>[2x]MLDSKLKAPVFTVRTQGREYGEFVLEPLERGFGVTLGNPLRRILLSSIPGTAVTSVYIEDVLHEFSTIPGVKEDVVEIILNLKELVVRFLNPSLQTVTLLLKAEGPKEVKARDFLPVADVEIMNPDLHIATLEEGGRLNMEVRVDRGVGYVPAEKHGIKDRINAIPVDAVFSPVRRVAFQVEDTRLGQRTDLDKLTLRIWTDGSVTPLEALNQAVEILREHLTYFSNPQAAAVAAPEEAKEPEAPPEQEEELDLPLEELGLSTRVLHSLKEEGIESVRALLALNLKDLKNIPGIGERSLEEIKEALEKKGFTLKE;> MEIKRFGRIREVIPLPPLTEIQVESYRRALQADVPPEKRENVGIQAAFRETFPIEEEDKGKGGLVLDFLEYRLGEPPFPQDECREKDLTYQAPLYARLQLIHKDTGLIKEDEVFLGHIPLMTEDGSFIINGADRVIVSQIHRSPGVYFTPDPARPGRYIASIIPLPKRGPWIDLEVEPNGVVSMKVNKRKFPLVLLLRVLGYDQETLARELGAYGELVQGLMDESVFAMRPEEALIRLFTLLRPGDPPKRDKAVAYVYGLIADPRRYDLGEAGRYKAEEKLGIRLSGRTLARFEDGEFKDEVFLPTLRYLFALTAGVPGHEVDDIDHLGNRRIRTVGELMTDQFRVGLARLARGVRERMLMGSEDSLTPAKLVNSRPLEAAIREFFSRSQLSQFKDETNPLSSLRHKRRISALGPGGLTRERAGFDVRDVHRTHYGRICPVETPEGANIGLITSLAAYARVDELGFIRTPYRRVVGGVVTDEVVYMTATEEDRYTIAQANTPLEGNRIAAERVVARRKGEPVIVSPEEVEFMDVSPKQVFSVNTNLIPFLEHDDANRALMGSNMQTQAVPLIRAQAPVVMTGLEERVVRDSLAALYAEEDGEVAKVDGNRIVVRYEDGRLVEYPLRRFYRSNQGTALDQRPRVVVGQRVRKGDLLADGPASENGFLALGQNVLVAIMPFDGYNFEDAIVISEELLKRDFYTSIHIERYEIEARDTKLGPERITRDIPHLSEAALRDLDEEGVVRIGAEVKPGDILVGRTSFKGESEPTPEERLLRSIFGEKARDVKDTSLRVPPGEGGIVVRTVRLRRGDPGVELKPGVREVVRVYVAQKRKLQVGDKLANRHGNKGVVAKILPVEDMPHL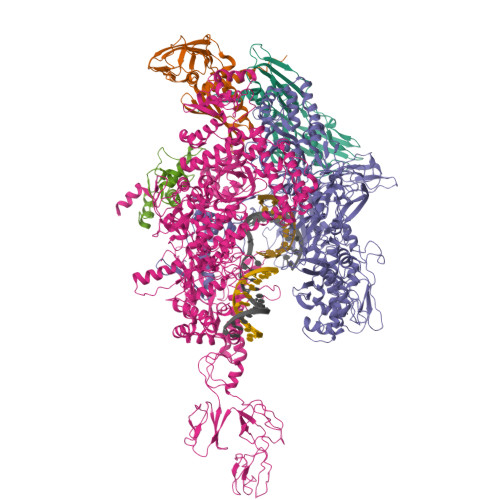PDGTPVDVILNPLGVPSRMNLGQILETHLGLAGYFLGQRYISPIFDGAKEPEIKELLAQAFEVYFGKRKGEGFGVDKREVEVLRRAEKLGLVTPGKTPEEQLKELFLQGKVVLYDGRTGEPIEGPIVVGQMFIMKLYHMVEDKMHARSTGPYSLITQQPLGGKAQFGGQRFGEMEVWALEAYGAAHTLQEMLTLKSDDIEGRNAAYEAIIKGEDVPEPSVPESFRVLVKELQALALDVQTLDEKDNPVDIFEGLASKR;> MKKEVRKVRIALASPEKIRSWSYGEVEKPETINYRTLKPERDGLFDERIFGPIKDYECACGKYKRQRFEGKVCERCGVEVTKSIVRRYRMGHIELATPAAHIWFVKDVPSKIGTLLDLSATELEQVLYFSKYIVLDPKGAILNGVPVEKRQLLTDEEYRELRYGKQETYPLPPGVDALVKDGEEVVKGQELAPGVVSRLDGVALYRFPRRVRVEYVKKERAGLRLPLAAWVEKEAYKPGEILAELPEPYLFRAEEEGVVELKELEEGAFLVLRREDEPVATYFLPVGMTPLVVHGEIVEKGQPLAEAKGLLRMPRQVRAAQVEAEEEGETVYLTLFLEWTEPKDYRVQPHMNVVVPEGARVEAGDKIVAAIDPEEEVIAEAEGVVHLHEPASILVVKARVYPFEDDVEVSTGDRVAPGDVLADGGKVKSDVYGRVEVDLVRNVVRVVESYDIDARMGAEAIQQLLKELDLEALEKELLEEMKHPSRARRAKARKRLEVVRAFLDSGNRPEWMILEAVPVLPPDLRPMVQVDGGRFATSDLNDLYRRLINRNNRLKKLLAQGAPEIIIRNEKRMLQEAVDALLDNGRRGAPVTNPGSDRPLRSLTDILSGKQGRFRQNLLGKRVDYSGRSVIVVGPQLKLHQCGLPKRMALELFKPFLLKKMEEKGIAPNVKAARRMLERQRDIKDEVWDALEEVIHGKVVLLNRAPTLHRLGIQAFQPVLVEGQSIQLHPLVCEAFNADFDGDQMAVHVPLSSFAQAEARIQMLSAHNLLSPASGEPLAKPSRDIILGLYYITQVRKEKKGAGLEFATPEEALAAHERGEVALNAPIKVAGRETSVGRLKYVFANPDEALLAVAHGIVDLQDVVTVRYMGKRLETSPGRILFARIVAEAVEDEKVAWELIQLDVPQEKNSLKDLVYQAFLRLGMEKTARLLDALKYYGFTFSTTSGITIGIDDAVIPEEKKQYLEEADRKLLQIEQAYEMGFLTDRERYDQILQLWTETTEKVTQAVFKNFEENYPFNPLYVMAQSGARGNPQQIRQLCGLRGLMQKPSGETFEVPVRSSFREGLTVLEYFISSHGARKGGADTALRTADSGYLTRKLVDVTHEIVVREADCGTTNYISVPLFQPDEVTRSLRLRKRADIEAGLYGRVLAREVEVLGVRLEEGRYLSMDDVHLLIKAAEAGEIQEVPVRSPLTCQTRYGVCQKCYGYDLSMARPVSIGEAVGIVAAQSIGEPGTQLTMRTFHTGGVAGAADITQGLPRVIELFEARRPKAKAVISEIDGVVRIEETEEKLSVFVESEGFSKEYKLPKEARLLVKDGDYVEAGQPLTRGAIDPHQLLEAKGPEAVERYLVEEIQKVYRAQGVKLHDKHIEIVVRQMMKYVEVTDPGDSRLLEGQVLEKWDVEALNERLIAEGKTPVAWKPLLMGVTKSALSTKSWLSAASFQNTTHVLTEAAIAGKKDELIGLKENVILGRLIPAGTGSDFVRFTQVVDQKTLKAIEEARKEAVEAKERPAARRGVKREQPGKQAHHHHHHHHHH;> MAEPGIDKLFGMVDSKYRLTVVVAKRAQQLLRHGFKNTVLEPEERPKMQTLEGLFDDPNAVTWAMKELLTGRLVFGENLVPEDRLQKEMERLYPVEREE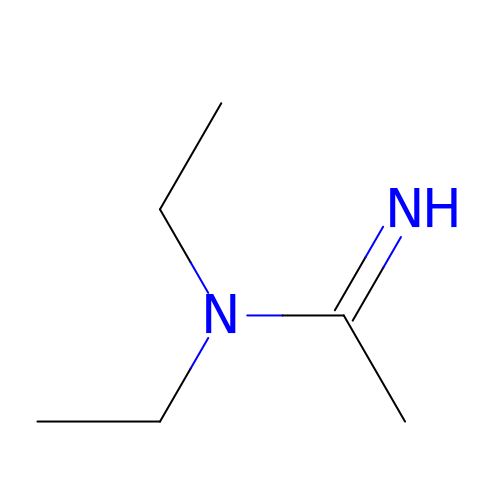(1Z)-N,N-diethylethanimidamide | C6 H14 N2 | RXSIKRLQGANXCL-SREVYHEPSA-N Interferon-γ-inducible protein (IP-10; CXCL10; 10 kDa) belongs to the CXC family of chemokines and is secreted by a variety of cell types. The biological activities of IP-10 are exerted by interactions with the G-protein-coupled receptor CXCR3 expressed on Th1 lymphocytes. IP-10 acts as an immunoinflammatory mediator in Th1-type inflammatory diseases, rheumatoid arthritis, cardiac allograft rejection, multiple sclerosis, atherosclerosis, sarcoidosis and prostate cancer. Oligomerization has been demonstrated to be an essential requirement for the biological function of IP-10.

Here, we present the crystal structure of mouse IP-10 at 2.5 Å resolution, which shows a novel oligomeric association. The final model contains four molecules in the asymmetric unit: A (residues 1–68), B (residues 1–67), C (residues 4–68) and D (residues 4–67). In each molecule, the N-terminal extended loop is stabilized by two disulfide bonds between conserved cysteines (9:36 and 11:53). In each of the two dimers, the β1 strands from each monomer associate to form a six-stranded β-sheet with two antiparallel α-helices lying on one face of the β-sheet. The dimers (A–D and B–C) are primarily stabilized by reciprocal interactions between opposing β1 strands. The main-chain hydrogen bonding at the interface is limited to reciprocal interactions between residues Leu27 and Ile29 (thus accounting for four hydrogen bonds) owing to the presence of Pro31, which disrupts the β-structure. In addition to the A–D and B–C dimers, another dimer is formed between molecules A and B in the mouse IP-10 structure. This results in a distinct tetrameric assembly that is formed by the association of two pseudosymmetrical dimers: A–D and B–C. The tetramer has an elongated structure with approximate dimensions of 90 × 40 Å2. Intermolecular contacts in the tetramer are through molecules A and B. The two molecules associate through their N-terminal loops in an antiparallel fashion such that their α-helices lie on one face of the β-strands, while the interacting N-terminal loops are on the back of the strands. The rotation axis parallel to the β-sheets and dissecting the A–B dimer relates chains A and B with a rotation angle of 179.1°, as calculated by LSQMAN. This is a novel association in which the tetramer consists of two six-stranded antiparallel β-sheets, with an antiparallel sheet formed by the N-­terminal regions between the two six-stranded β-­sheets and all four helices lying on one face of the β-sheet. The solvent-accessible area at the interface in the dimer is reduced by 1770 Å2, which is higher than the buried surface area of the pseudosymmetrical dimers A–D and B–C (1280 and 1170 Å2, respectively).

>IPLARTVRCNCIHIDDGPVRMRAIGKLEIIPASLSCPRVEIIATMKKNDEQRCLNPESKTIKNLMKAF[4x]> GPMPGLPIKLRVEKAYPEDVGKRAVRMDK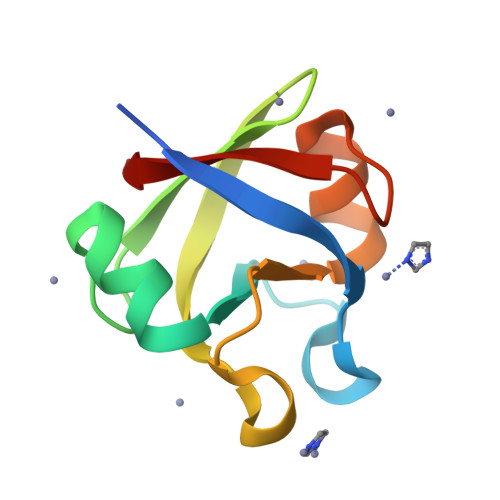ASRDRIGVSEGDLVKITGSKTTVARVLPAKKEDVGKGIVRMDKYERQNAGASVGEPVEVDRAE> PVWGCASTRGRSAEMEDASAAVPRFADVPVRLLASRRDLDALGLDADALRLPAHLFGVFDGHGGAEVANYCRERIHVVLSAALARLGKNLGEMGEVDMKEHWDDVFTKCFQRVDDEVSGRVTRVVNGGGEVRSEPVTAENVGSTAVVALVCSSHVVVANCGDSRIVLCRGKEPVALSIDHKPDRKDERARIEAQGGKVIQWNGYRVFGMLAMSRSIGDRYLKPFVIPKPEVMVVPRAKDDDCLILASDGLWDVVSNEEAC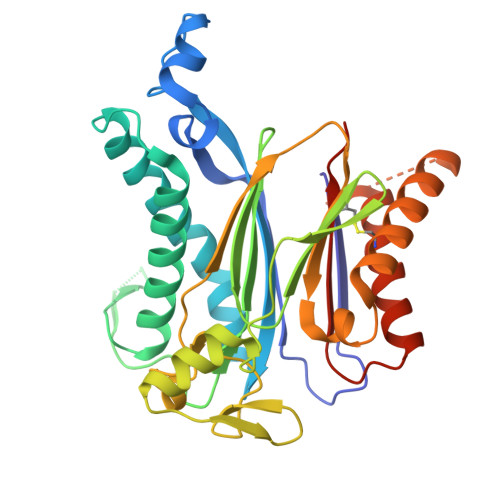KVARRQILLWHKNNGAASPLSDEGEGSTDPAAQAAADYLMRLALKKGSEDNITVIVVDLKPRKKLKN>[3x]MWIIEAEGDILKGKSRILFPGTYIVGRNVSDDSSHIQVISKSISKRHARFTILTPSEKDYFTGGPCEFEVKDLDTKFGTKVNEKVVGQNGDSYKEKDLKIQLGKCPFTINAYWRSMCIQFDNPEMLSQWASNLNLLGIPTGLRDSDATTHFVMNRQAGSSITVGTMYA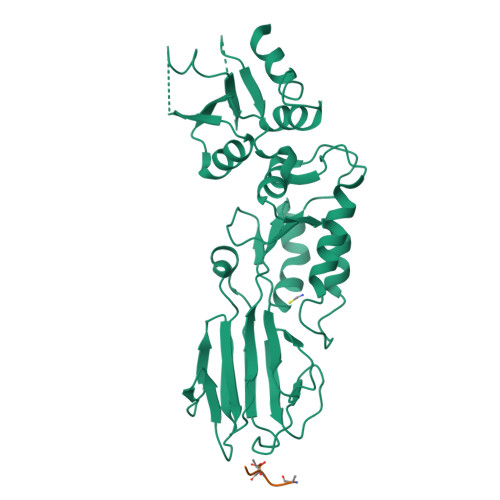FLKKTVIIDDSYLQYLSTVKESVIEDASLMPDALECFKNIIKNNDQFPSSPEDCINSLEGFSCAMLNTSSESHHLLELLGLRISTFMSLGDIDKELISKTDFVVLNNAVYDSEKISFPEGIFCLTIEQLWKIIIERNSRELISKEIERLKYATLVPR;> IQELDSTTDEDEI> MAQETYFYGQGEIDAAPIVNGVLGKWRWIQDVSAMSIQLAVEKVEHKESYSGQKALVRSFPIGKTATVNITLHSIGPDNLALTLYGKVVAKAAGSVTGEVLPADLVAGDVIR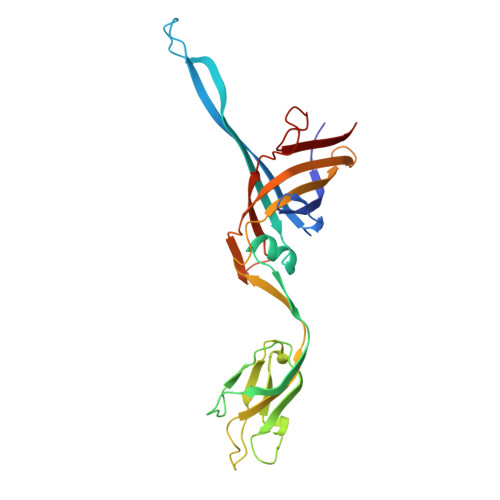LANFGVSELVITDSASSPAPLDPQYYALRADGAYGEVQLLGLPTPAPTQPFKAAYEYAATKQVGMFTAPQPTVALRYKGINLAEGGAPVIVELYKVATDPLQELALISDGNTVAGMQISGGILLDTSKPDTGDLGRFGRIIQLG>[4x]PMKTILVTGGSGFLGRRLVSHLSKNYTVVAPTHGELDLTDREKIISEVTKINPQIIIHTAAISNTGLCEQNPELSESINLNGTKYLAEAASKINSKLIFCSSDQIYNGNAEKGPLSEDIDVHPVNVYGKHKLEAERKLQEILPTSVSLRLTWMYDHPSSKIPQHKNLPIMLLEAKEKNVPFVTTVNEYRAITFVGEVVENIEKTFELPGGVYNYG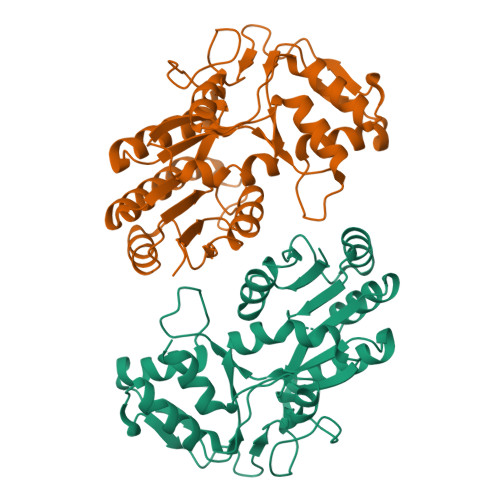ASNTSNSYETYKEIAKIMDVPENLVENDTNRFKAQARNISMNIQKIEKHGIHFSNTVDGFSKMYKSFSNSE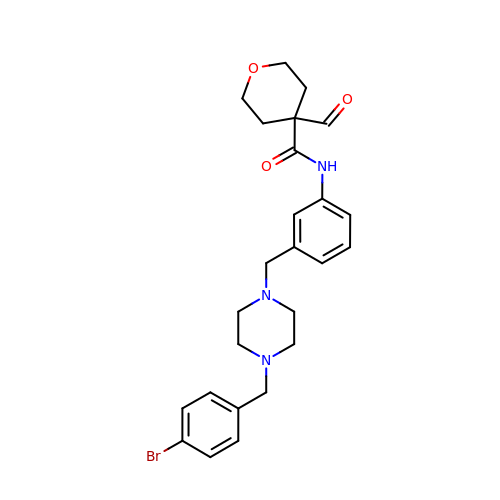~{N}-[3-[[4-[(4-bromophenyl)methyl]piperazin-1-yl]methyl]phenyl]-4-methanoyl-oxane-4-carboxamide | C25 H30 Br N3 O3 | PPXXFRMHSKGYSK-UHFFFAOYSA-N>VPANAVTESDPAAVALKYHRDAASSERVAAAR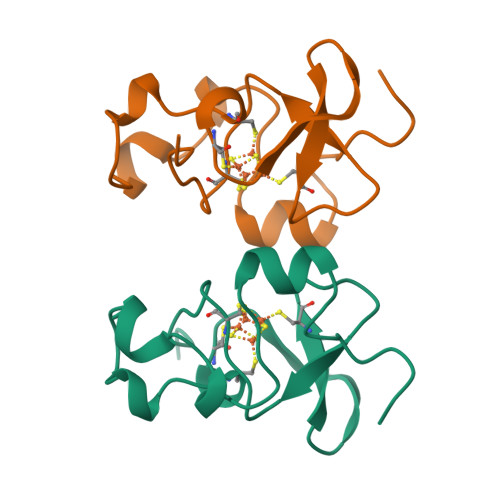PGLPPEEQHCENCQFMNPDSAAADWKGCQLFPGKLINLSGWCASWTLRAG[3x]>MSASIPDIKLSSGHLMPSIGFGCWKLANATAGEQVYQAIKAGYRLFDGAEDYGNEKEVGDGVKRAIDEGLVKREEIFLTSKLWNNYHDPKNVETALNKTLADLKVDYVDLFLIHFPIAFKFVPIEEKYPPGFYCGDG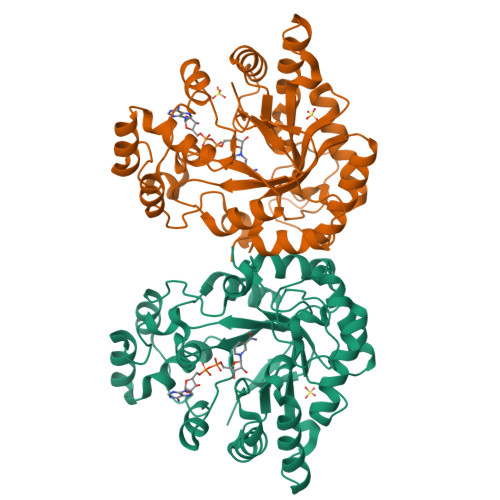NNFVYEDVPILETWKALEKLVAAGKIKSIGVSNFPGALLLDLLRGATIKPAVLQVEHHPYLQQPKLIEFAQKAGVTITAYSSFGPQSFVEMNQGRALNTPTLFAHDTIKAIAAKYNKTPAEVLLRWAAQRGIAVIPRSNLPERLVQNRSFNTFDLTKEDFEEIAKLDIGLRFNDPWDWDNIPIFV[4x]> MALRGTVTDFSGFDGRADAEVLRKAMKGLGTDEDSILNLLTARSNAQRQQIAEEFKTLFGRDLVNDMKSELTGKFEKLIVALMKPSRLYDAYELKHALKGAGTDEKVLTEIIASRTPEELRAIKQAYEEEYGSNLEDDVVGDTSGYYQRMLVVLLQANRDPDTAIDDAQVELDAQALFQAGELKAGTDEEKFITILGTRSVSHLRRVFDKYMTISGFQIEETIDRETSGNLENLLLAVVK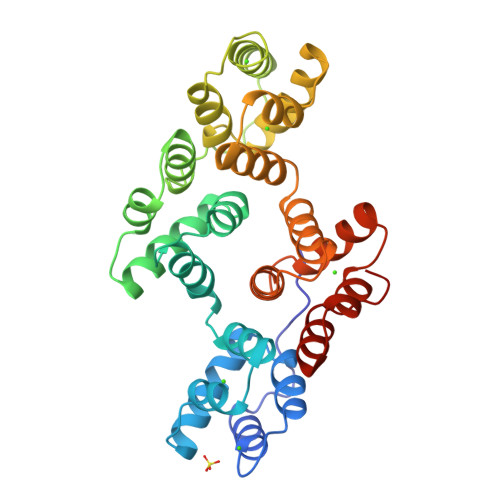SIRSIPAYLAETLYYAMKGAGTDDHTLIRVIVSRSEIDLFNIRKEFRKNFATSLYSMIKGDTSGDYKKALLLLCGGEDD>GSHMEAVQNRIVEAAERVPGVRGVIHLRARYVGQDIWADMIIGVDPENTVEQAEEICEAVQAAVCGKIRRIESLHVSAHAREIGDTTKPSFSDQPLSFDEVMLSKVDN[4x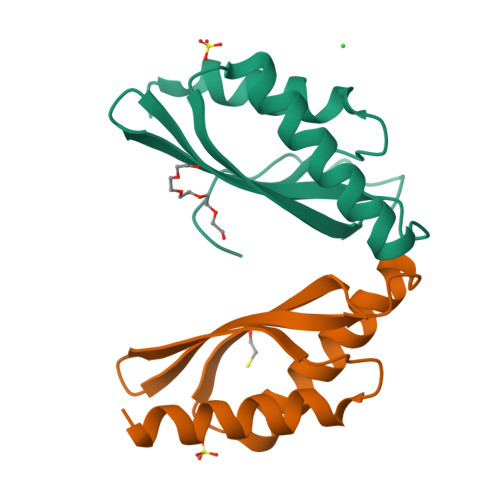]> GSKKKIDILL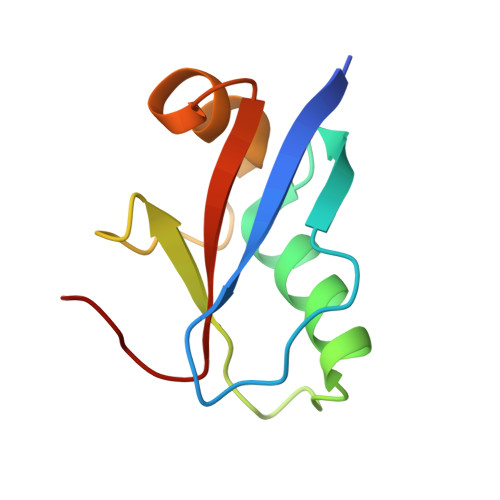KAVGDTPIMKTKKWAVERTRTIQGLIDFIKKFLKLVASEQLFIYVNQSFAPSPDQEVGTLYECFGSDGKLVLHYCKSQAWG> MRVNNCLTPQELEAYGISDVHDIVYNPSYDLLYQEELDPSLTGYERGVLTNLGAVAVDTGIFTGRSPKDKYIVRDDTTRDTFWWADKGKGKNDNKPLSPETWQHLKGLVTRQLSGKRLFVVDAFCGANPDTRLSVRFITEVAWQAHFVKNMFIRPSDEELAGFKPDFIVMNGAKCTNPQWKEQGLNSENFVAFNLTERMQLIGGTWYGGEMKKGMFSMMNYLLPLKGIASMHCSANVGEKGDV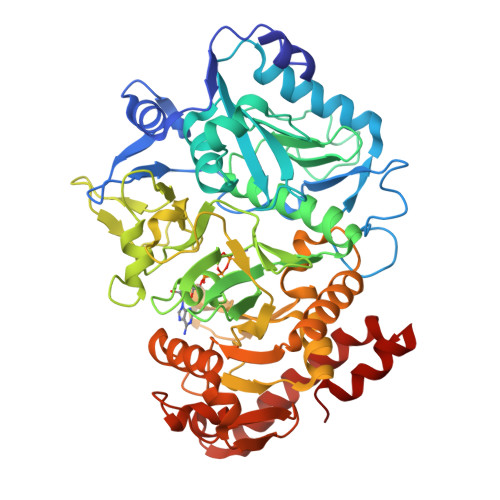AVFFGLAGTGKTTLSTDPKRRLIGDDEHGWDDDGVFNFEGGCYAKTIKLSKEAEPEIYNAIRRDALLENVTVREDGTIDFDDGSKTENTRVSYPIYHIDNIVKPVSKAGHATKVIFLTADAFGVLPPVSRLTADQTQYHFLSGFTAKLAGTERGITEPTPTFSACFGAAFLSLHPTQYAEVLVKRMQAAGAQAYLVNTGWNGTGKRISIKDTRAIIDAILNGSLDNAETFTLPMFNLAIPTELPGVDTKILDPRNTYASPEQWQEKAETLAKLFIDNFDKYTDTPAGAALVAAGPKL2-(2,3-dihydro-1-benzofuran-5-yl)-N-[2-(piperazin-1-yl)phenyl]-1,3-thiazole-4-carboxamide | C22 H22 N4 O2 S | 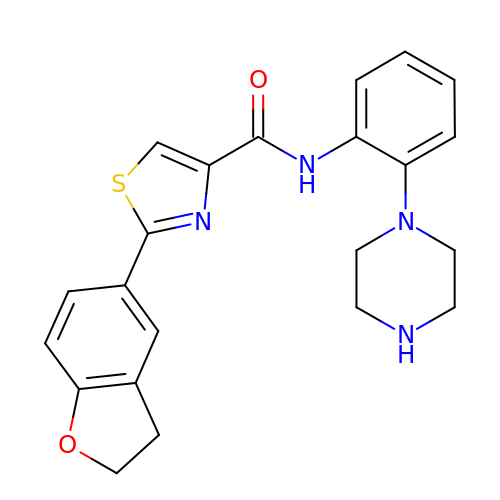WRGSHXQBWJUKQD-UHFFFAOYSA-N>[4x]GSHMKIR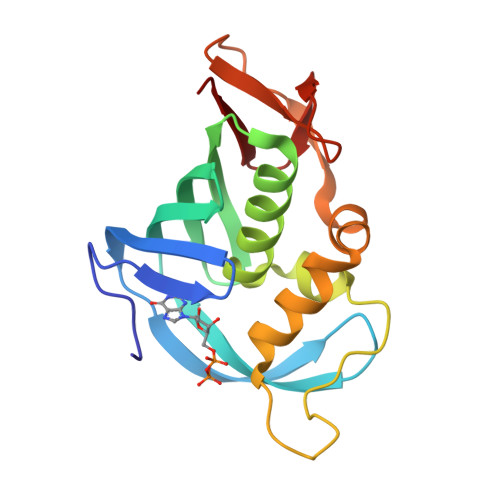QRQRFGRLELKRISGRGFKNDEEILIGNGTIQKIGIWDGEEEFHVRCGECRGILKKSKMKLEKLLINSAKKEDMRDLIILCMVFSQDTRMFQGVRGEINFLNRAGQLLSPMYQLQRYFLNRSSDLFDQWGYEESPKASELHGINESMNASDYTLKGVVVTKN>[4x]SANDKQYISYNNVHQLCQVSAERIKNFKPDLIIAIGGGGFIPARILRTFLKEPGVPTIRIFAIILSLYEDLNSVGSEVEEVGVKVSRTQWIDYEQCKLDLVGKN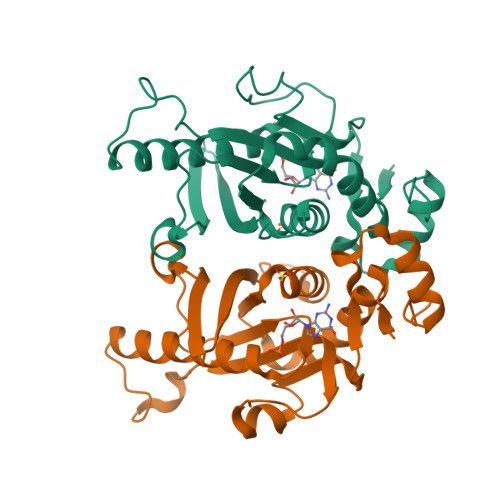VLIVDEVDDTRTTLHYALSELEKDAAEQAKAKGIDTEKSPEMKTNFGIFVLHDKQKPKKADLPAEMLNDKNRYFAAKTVPDKWYAYPWESTDIVFHTRMAIEQGNDIFIPEQEHKQ>MKSTSDLFNEIIPLGRLIHMVNQKKDRLLNEYLSPLDITAAQFKVLSSIRSAASITPVELKKVLSVDLGALTRMLDRLVSKGWVERLPNPNDKRGVLVKLTTGGAAIS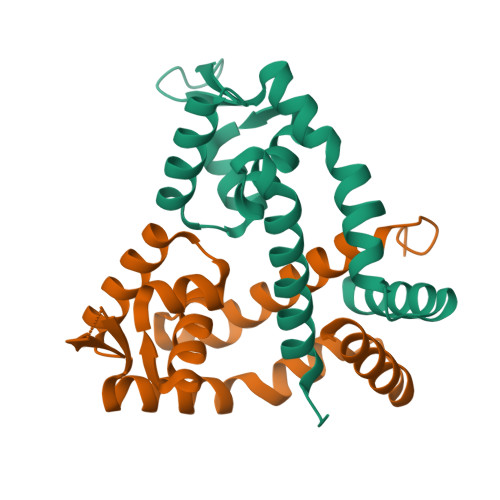EQSHQLVGQDLHQELTKNLTADEVATLEYLLKKVLP[2x]> SIYNSFYVYCKGPCQRVQPGKLRVQCSTCRQATLTLTQGPSCWDDVLIPNRMSGECQSPHCPGTSAEFFFKCGAHPTSDKETSVALHLIATNSRNITCITCTDVRSPVLVFQCNSRHVICLDCFHLYCVTRLNDRQFVHDPQLGYSLPCVAGCPNSLIKELHHFRILGEEQYNRYQQYGAEECVLQMGGVLCPRPGCGAGLLPEPDQRKVTCEGGNGLGCGFAFCRECKEAYHEGECSAVFEASGT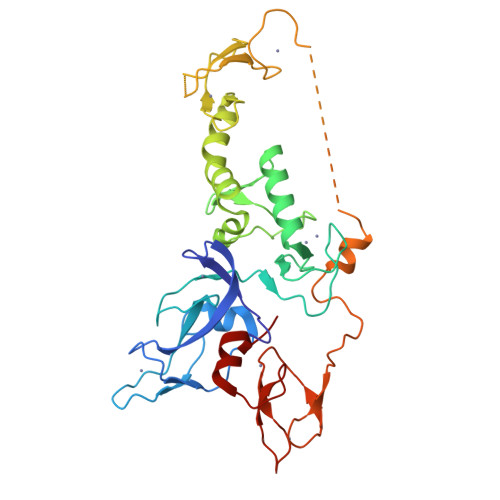TTQAYRVDERAAEQARWEAASKETIKKTTKPCPRCHVPVEKNGGCMHMKCPQPQCRLEWCWNCGCEWNRVCMGDHWFDV> MSKLTTGSFSIEDLESVQITINNIVGAAKEAAEEKEKELVNAGPTLFPGLEGYRDDWNFKLLDRYEPVITPMCDQCCYCTYGPCDLSGNKRGACGIDMKGHNGREFFLRVITGTACHAAHGRHLLDHLIEKYGEDLPLTLGQSNVLTPNITISTGLSPKTLGEVKPAMEYVEEQLTQLLATVHAGQESAEIDYDSKALFSGSLDHVGMEISDIVQVAAYDFPKADPEAPLVEIGMGTIDKSKPFLCVIGHNVAGVTYMMDYMEDNNLTDKMEIAGLCCTAIDLTRYKEADRRPPYAKVIGSMSKELKVIRSGMPDVIVVDEQCVRGDIVPEAQKLKIPVIASNPKIMYGLPNRTDADVDETMEELKSGKIPGCVMLDYDKLGELCVRLTMEMAPIRDAAGITALPTDEELVNMVAKCADCGACLLACPEEIDIPEAMGFAKKGDFSYFEEIHDTCIGCRRCEQVCKKEIPILNVIEKIAQKQIAEEKGLMRAGRGQVSDAEIRAEGLNLVMGTTPGIIAIIGCPNYAGGTKDVYYIAEEFLKR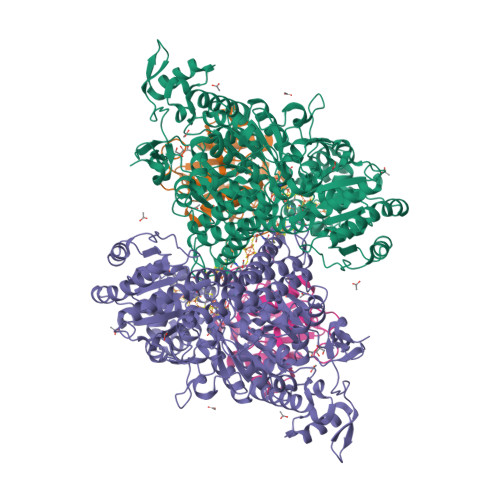NFIVVTTGCGAMDIGMFKDADGKTLYERFPGGFQCGGLANIGSCVSNAHITGAAEKVAAIFAQRTLEGNLAEIGDYILNRVGACGLAWGAFSQKASSIGTGCNIFGIPAVLGPHSSKYRRALIAKTYEEDKWKVYDARNGQEMPIPPAPEFLLTTAETWQEAIPMMAKACIRPSDNSMGRAIKLTHWMELHKKYLGGKEPEDWWKFVRTEADLPLATREALLKELEKEHGWEIDWKRKKIISGPKIKFDVSAQPTNLKRLCKEA;> MVDTTKNTKLFTSYGVNTSKAVSPEMAAKIISKAKRPLLMVGTLALDPELLDRVVKISKAANIPIAATGSSLAVLADKDVDAKYINAHMLGFYLTDPKWPGLDGNGNYDMIITIGFKKFYINQVLSAAKNFSNLKTIAIERGYIQNATMSFGNLSKADHYAALDELINAL> SFREQDIYLPIANVARIMKNAIPQTGKIAKDAKECVQECVSEFISFITSEASERCHQEKRKTINGEDILFAMSTLGFDSYVEPLKLYLQ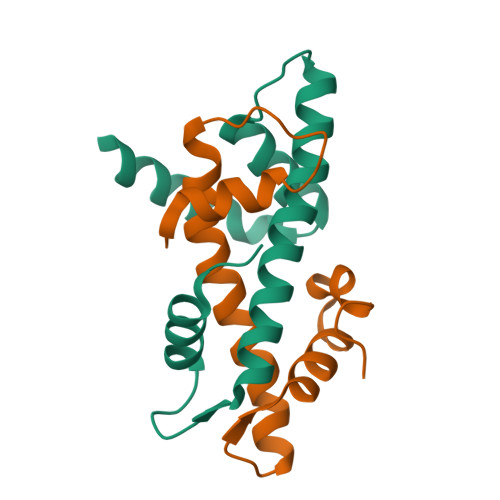KFRE;> GSHMEEIRNLTVKDFRVQELPLARIKKIMKLDEDVKMISAEAPVLFAKAAQIFITELTLRAWIHTEDNKRRTLQRNDIAMAITKFDQFDFLIDIVPR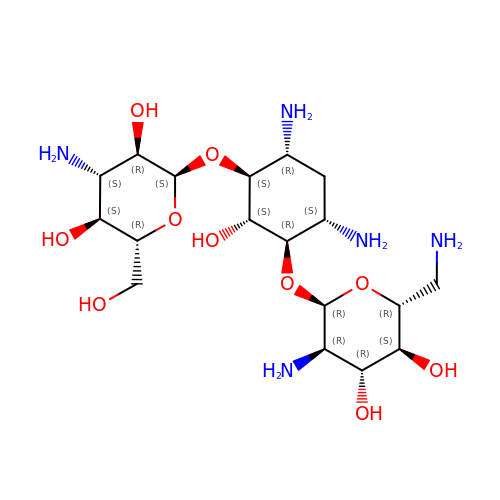(1R,2S,3S,4R,6S)-4,6-DIAMINO-3-[(3-AMINO-3-DEOXY-ALPHA-D-GLUCOPYRANOSYL)OXY]-2-HYDROXYCYCLOHEXYL 2,6-DIAMINO-2,6-DIDEOXY-ALPHA-D-GLUCOPYRANOSIDE | C18 H37 N5 O10 | SKKLOUVUUNMCJE-FQSMHNGLSA-N>GPHMEDEAYFIAKEILATERTYLKDLEVITVWFRSVLIKEEAMPAALMALLFSNIDPVYEFHRGFLHEVEQRLALWEGPSSAHLKGDHQRIGDILLRNMRQLKEFTSYFQRHDEVLTELEKATKHCKKLEAVYKEFELQKVCYLPLNTFLLKPVQRLVHYRLLLSRLCAHYSPGHRDYADCHEALKAITEVTTELQQSLTRLENLQKLTELQRDLVGVENLIAPGREFIREGCLHKLTKKGLQQRMFFLFSDMLLYTSKSVTGASHFRIRGFLPLRGMLVEESENEWSVLHCFTIYAAQKTIVVAASTRLEKEKWMQDLNAAIQAAKTIGDSPPVLLGGPVYTRTPRSSDEVSLEESEDGRGNRGSLEGNSQHRANTTMHVCWYRNTSVSRADHSAAVENQLSGYLLRKFKNSNGWQKLWVVFTNFCLFFYKTHQDDYPLASLPLLGYSVSLPREADSIHKDYVFKL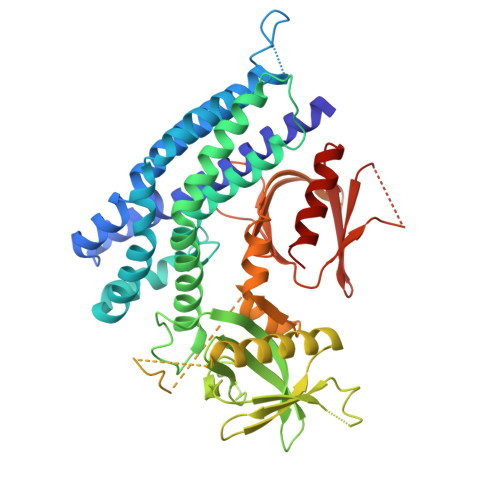QFKSHVYFFRAESKYTFERWMDVIKRASSSPGRP[2x]> MATSRYEPVAEIGVGAYGTVYKARDPHSGHFVALKSVRVPNGEEGLPISTVREVALLRRLEAFEHPNVVRLMDVCATSRTDREIKVTLVFEHVDQ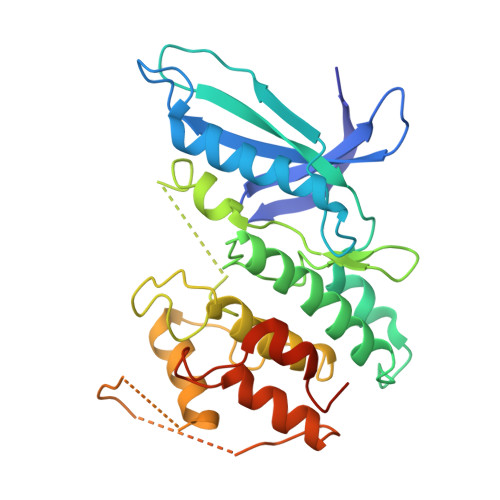DLRTYLDKAPPPGLPAETIKDLMRQFLRGLDFLHANCIVHRDLKPENILVTSGGTVKLADFGLARIYSYQMALFPVVVTLWYRAPEVLLQSTYATPVDMWSVGCIFAEMFRRKPLFCGNSEADQLGKIFDLIGLPPEDDWPRDVSLPRGAFPPRGPRPVQSVVPEMEESGAQLLLEMLTFNPHKRISAFRALQHSYLHKDEGNPEHHHHHH>AETVSFNFNSFSEGNPAINFQGDVTVLSNGNIQLTNLNKVNSVGRVLYAMPVRIWSSATGNVASFLTSFSFEMKDIKDYDPADGIIFFIAPEDTQIPAGSIGGGTLGVSDTKGAGHFVGVEFDTYSNSEYNDPPTDHVGIDVNSVDSVKTVPWNSVSGAVVKVTVIYDSSTKTLSVAVTNDNGDITTIAQVVDLKAKLPERVKFGFSASGSLGGRQIHLIRSWSFTSTLITTTR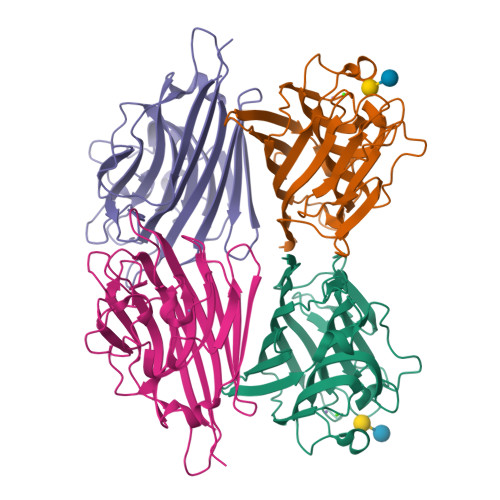RS[8x]> MSEQSICQARASVMVYDDTSKKWVPIKPGQQGFSRINIYHNTASSTFRVVGVKLQDQQVVIN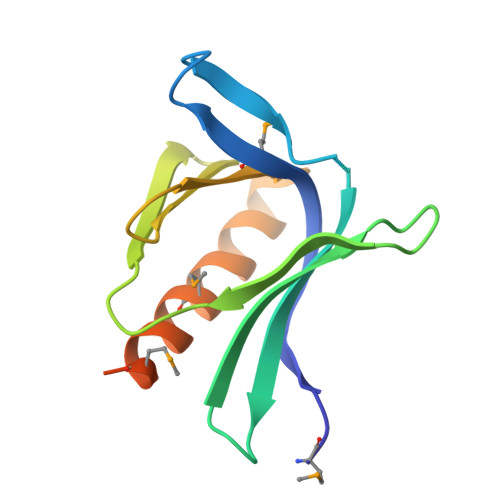YSIVKGLKYNQATPTFHQWRDARQVYGLNFASKEEATTFSNAMLFALNIMNSQEGGPSTQRQVQNGPS>TAPSQVLKIRRPDDWHLHLRDGDMLKTVVPYTSEIYGRAIVMPNLAPPVTTVEAAVAYRQRILDAVPAGHDFTPLMTCYLTDSLDPNELERGFNEGVFTAAKLYPANAVTNSSHGVTSVDAIMPVLERMEKIGMPLLVHGEVTHADIDIFDREARFIESVMEPLRQRLTALKVVFEHITTKDAADYVRDGNERLAATITPQHLMFNRNHMLVGGVRPHLYCLPILKRNIHQQALRELVASGFNRVFLGTDSAPHARHRKESSCGCAGCFNAPTALGSYATVFEEMNALQHFEAFCSVNGPQFYGLPVNDTFIELVREEQQVAE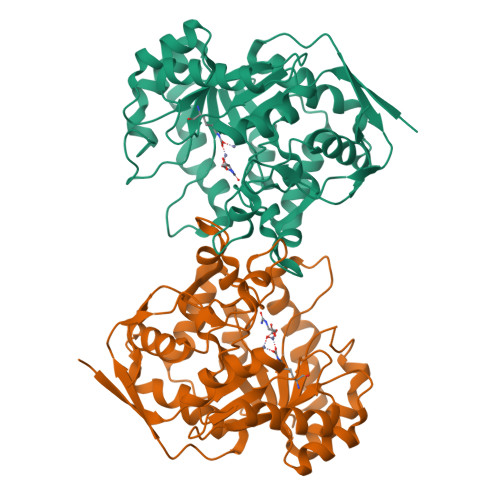SIALTDDTLVPFLAGETVRWSVKQ[2x]>AETSSATTAQQMPSLAPMLEKVMPSVVSINVEGSTTVNTPRMPRNFQQFFGDDSPFCQEGSPFQSSPFCQGGQGGNGGGQQQKFMALGSGVIIDADKGYVVTNNHVVDNATVIKVQLSDGRKFDAKMVGKDPRSDIALIQIQNPKNLTAIKMADSDALRVGDYTVAIGNPFGLGETVTSGIVSALGRSGLNAENYENFIQTDAAINRGNAGGALVNLNGELIGINTAILAPDGGNIGIGFAIPSNMVKNLTSQMVEYGQVKRGELGIMGTELNSELAKAMKVDAQRGAFVSQVLPNSSAAKAGIKAGDVITSLNGKPISSFAALRAQVGTMPVGSKLTLGLLRDGKQVNVNLELQQSSQNQV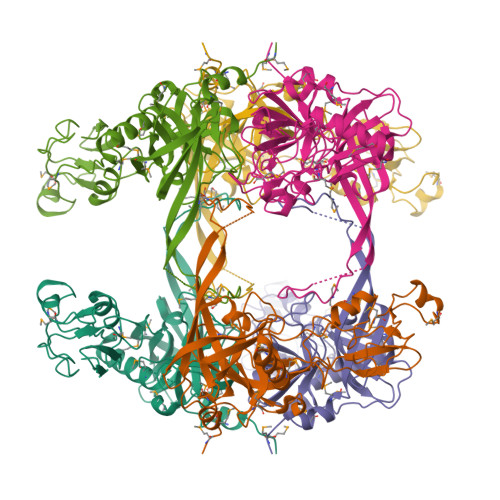DSSSIFNGIEGAEMSNKGKDQGVVVNNVKTGTPAAQIGLKKGDVIIGANQQAVKNIAELRKVLDSKPSVLALNIQRGDSTIYLLMQ[2x]> GPLGSPS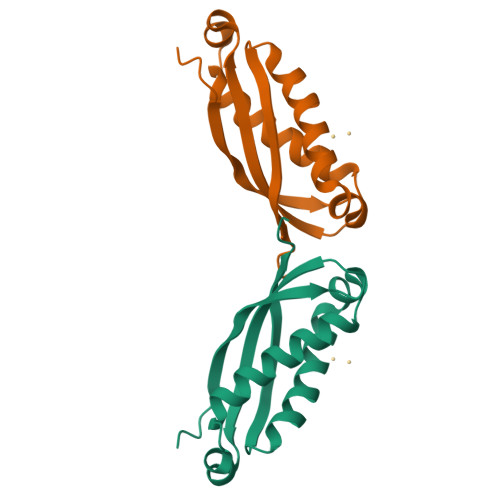TDSAAKVDMRTISFDIPPQEVLTKDSVTISVDGVVYYRVQNATLAVANITNADSATRLLAQTTLRNALGTKNLSQILSDREEIAHHMQSTLDDATDDWGIKVERVEIKDVKLPVQLQRAMAAEAEA(2R,4S)-2-methyl-2,3,3,4-tetrahydroxytetrahydrofuran 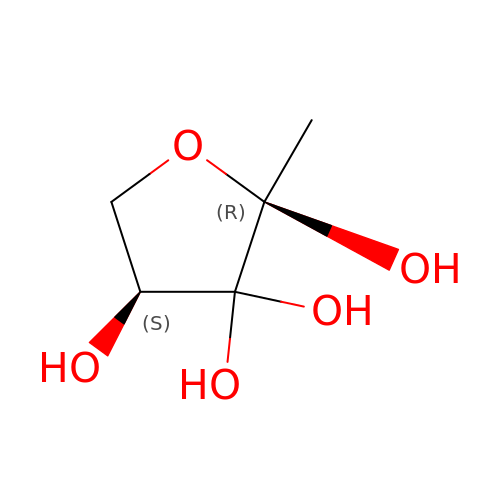| C5 H10 O5 | BVIYGXUQVXBHQS-IUYQGCFVSA-N A number of enzymes, termed fructosyl amino acid oxidase (FAOX), have reactivity for fructosyl amino acids as major substrates. Some of these enzymes, which also exhibit reactivity for fructosyl dipeptides as F-VH are specifically termed fructosyl peptide oxidase (FPOX). AnFPOX-15, which featured 11 amino acid replacements in AnFPOX-1 exhibited significant F-VH oxidation activity, whereas reactivity for longer fructosyl peptides such as fructosyl tripeptide (F-3P, Fru-VHL), fructosyl tetrapeptide (F-4P, Fru-VHLT) and F-6P was never observed. The overall structure of AnFPOX-15 consisted of two domains: an oxidoreductase FAD-binding domain with the topology of an incomplete anti-parallel β-barrel (two β-sheets with eight β-strands) and four α-helices at one side of the β-barrel; and a catalytic domain with two β-sheets (eight or two β-strands), and two long α-helices (helix 2 and 3) that locate at each side of the sheets, and some short helices.

Therefore, we initially attempted to determine the crystal structure of AnFPOX-15 for detailed rational design. The refined models comprised 431 residues for a protein molecule in an asymmetric unit, although the enzyme consisted of 438 residues. All amino acid residues (P3-R433), except for the N-terminal residues (M1 and A2), could be assigned to the 2Fo-Fc map; however, the electron-density map for residues S297-I303 and H309-P313 were relatively ambiguous. The structure of AnFPOX-15 resembled the known structures of other FPOX enzymes. Recently, the crystal structures of group I FPOX, namely Eupenicillium terrenum FPOX (EtFPOX)17 and Phaeosphaeria nodorum FPOX (PnFPOX), were reported. They both shared high amino acid sequence identity with AnFPOX-15 as well as showed quite low rmsd value compared with AnFPOX-15 (0.80 Å and 1.12 Å, respectively), suggesting their structural similarity. No significant structural difference was observed between the ligand-free AnFPOX-15 and AnFPOX-15/FSA (rmsd = 0.46 Å for 429 Cα atoms).

> MAPRANTKIIVVGGGGTMGSSTALHLLRAGYTPSNITVLDTYPIPSAQSAGYDLNKIFGIRLRNKPDLQLYLEALDMWKNDPLFKPFFHNVGQMDVSSTEEGIKKLRMRYQSLLDAGIGLEKTNFLLESEDEILAKAPHFTREQIKGWKGLFCGDGGWLAAAKAINAIGQFLKEQGVKFGFGEAGTFKKPLFADADEKTCIGVETVDGTKYYADKVVLAAGAWSSTLVDLEEQCVSKAWVFAHIQLTPAEAAAYKNTPVIYDGDYGFFIEPDENGIIKVCDEFPGFTHFKMHQPYGSPVPKLISVPRSHAKHPTDTYPHASEVTIKKAINRFLPRFNDKELFNRAMCWCTDTADANLLVCEHPRWKGFYLATGDSGHSFKLLPNIGKHVVELLEGRLESVFKDAWRWRPGSGDALKSRRAAPAKDLADMPGWRNEAKM>[2x]GAGSTAGKVIKCKAAVLWEEKKPFSIEEVEVAPPKAHEVRIKMVATGICRADDHVVSGTLVTPLPVIAGHEAAGIVESIGEGVTTVRPGDKVIPLFTPQCGKCRVCKHPEGN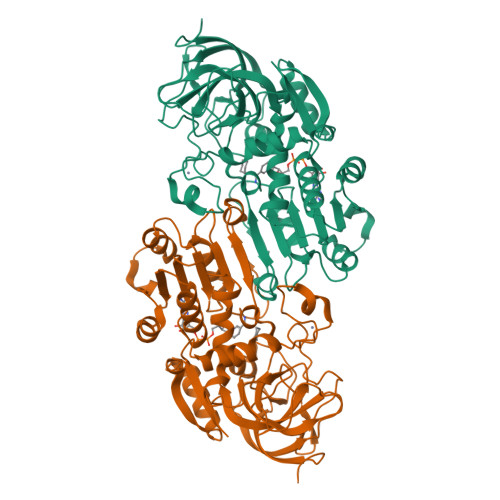FCLKNDLSMPRGTMQDGTSRFTCRGKPIHHFLGTSTFSQYTVVDEISVAKIDAASPLEKVCLIGCGFSTGYGSAVKVAKVTQGSTCAVFGLGGVGLSVIMGCKAAGAARIIGVDINKDKFAKAKEVGATECVNPQDYKKPIQEVLTEMSNGGVDFSFEVIGRLDTMVTALSCCQEAYGVSVIVGVPPDSQNLSMNPMLLLSGRTWKGAIFGGFKSKDSVPKLVADFMAKKFALDPLITHVLPFEKINEGFDLLRSGESIRTILTF1,3-BISPHOSPHOGLYCERIC 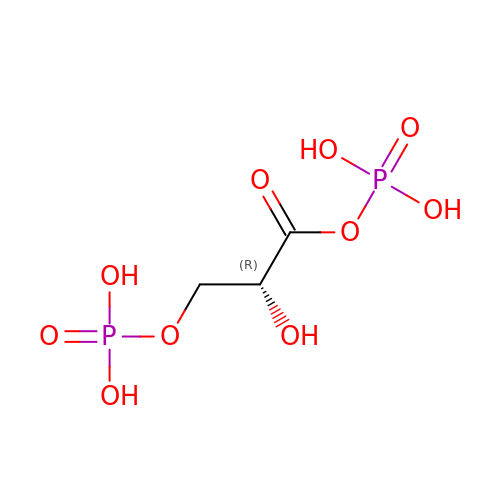ACID | C3 H8 O10 P2 | LJQLQCAXBUHEAZ-UWTATZPHSA-N>MNSPISPIETVPVKLKPGMDGPKVKQWPLTEEKIKALVEICTEMEKEGKISKIGPENPYNTPVFAIKKKDSTKWRKLVDFRELNKRTQDFWEVQLGIPHPAGLKKNKSVTVLDVGDAYFSVPLDEDFRKYTAFTIPSINNETPGIRYQYNVLPQGWKGSPAIFQSSMTKILEPFRKQNP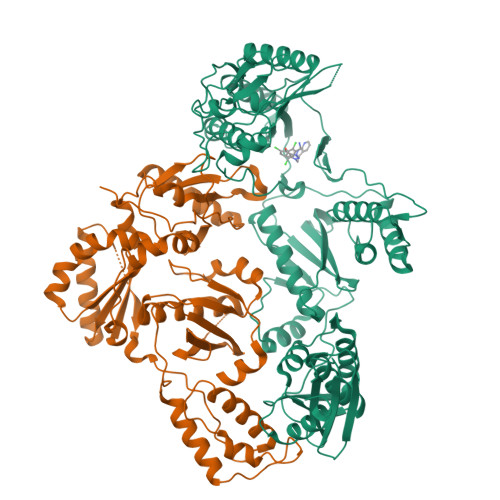DIVIYQYMDDLYVGSDLEIGQHRTKIEELRQHLLRWGLTTPDKKHQKEPPFLWMGYELHPDKWTVQPIVLPEKDSWTVNDIQKLVGKLNWASQIYPGIKVRQLCKLLRGTKALTEVIPLTEEAELELAENREILKEPVHGVYYDPSKDLIAEIQKQGQGQWTYQIYQEPFKNLKTGKYARMRGAHTNDVKQLTEAVQKITTESIVIWGKTPKFKLPIQKETWETWWTEYWQATWIPEWEFVNTPPLVKLWYQLEKEPIVGAETFYVDGAANRETKLGKAGYVTNRGRQKVVTLTDTTNQKTELQAIYLALQDSGLEVNIVTDSQYALGIIQAQPDQSESELVNQIIEQLIKKEKVYLAWVPAHKGIGGNEQVDKLVSAGIRKVL[2x]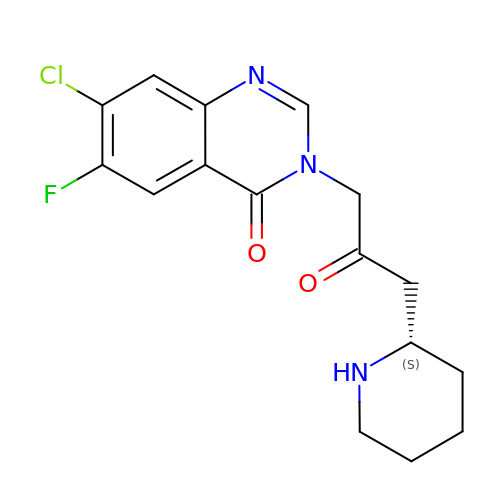7-chloro-6-fluoro-3-{2-oxo-3-[(2S)-piperidin-2-yl]propyl}quinazolin-4(3H)-one | C16 H17 Cl F N3 O2 | LZMOBHASNVDDQN-JTQLQIEISA-N> LTFEQYWAQL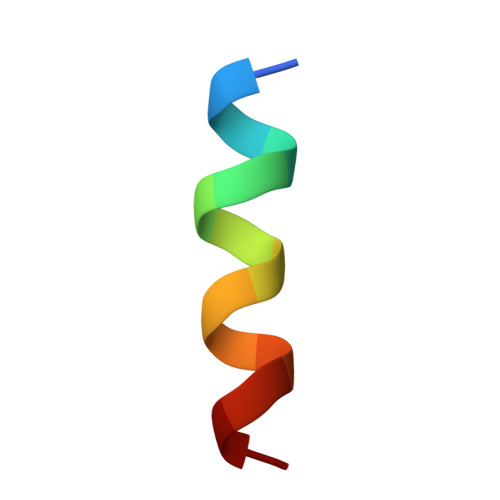ESAA>[9x]LDPEERYEHQLRQLNDMG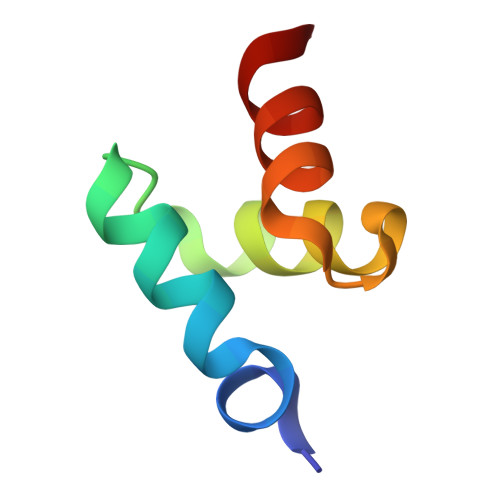FFDFDRNVAALRRSGGSVQGALDSLLNG Previously, the biosynthetic pathway of the immunosuppressive agent caerulomycin A (CRM A) from the marine actinomycete Actinoalloteichus cyanogriseus WH1-2216-6 has been identified, and the critical role of the (S)-selective ω-transaminase CrmG in the biosynthesis of CRM A has been reported. CrmG catalyzes amino acceptor caerulomycin M (CRM M) transformation to caerulomycin N (CRM N). Moreover, the activity of CrmG is insensitive to inhibition from ketone α-ketoglutarate or pyruvate.

The crystal structures of CrmG in complex with amino donor l-Gln, l-Glu, or l-Ala in P1 space group were determined to resolution 2.35, 2.25, and 2.20 Å, respectively. For these three crystal structures, each asymmetric unit contains two dimers. In the structures of CrmG with l-Glu or l-Ala, clear electron density was observed between the N atoms of those amino donors and the C4′ atom of PLP, indicating that we have captured the external aldimine for these amino acids. In the structure of CrmG with PLP-Glu, γ-carboxylate of the l-Glu portion not only forms a hydrogen bond with S372′ but also forms an additional salt bridge with K210. Based on these three crystal structures, amino donors l-Glu, l-Gln, and l-Ala exhibit strong, moderate, and weak binding to CrmG, respectively, due to side chain differences. These corroborate well with our kinetic data that, Km value for l-Glu, l-Gln, and l-Ala toward CrmG is 80.02, 182.70, and 405.10 μM, respectively. Moreover, in the case of l-Glu, which forms stronger interactions with the active site of CrmG than l-Ala, the corresponding by-product α-ketoglutarate also exhibits very weak inhibitory potential with a Ki value of 145.9 mM. The energy profile for CrmG catalyzing l-Glu deamination was calculated based on the crystal structures of PLP-bound CrmG and l-Glu-bound CrmG; the energy profile for CrmG catalyzing CRM M amination was calculated based on structures of PMP-bound CrmG and CRM M-bound CrmG. CrmG catalyzing l-Glu deamination is an exothermic reaction with calculated reaction enthalpy of −33.5 kcal/mol, and CRM M amination is endothermic with calculated reaction enthalpy of 11.5 kcal/mol.

>[4x]MTHPSGEPVYADAVLNGWLTSMGLGVEYVRAEGNTVYYLDDEGREVPVLDHACGFGSLIFGHNHPEIIAHAKAALDAGTVVHAQLSRQPRANQISRILNDIMRRETGRDDRYNAIFANSGAEANEICMKHAELERQERITALFAEIDAELDTAREALTTGTATLDTASLPLVGGGAGDVDGVIADIHRHNDERRAERPLFLTLDGSFHGKLVGSIQLTQNEPWRTPFTALSSPARFLPADEPELIGKIVEDERRSVLTLSLDKDTVRVVERDFPVVAAIFVEPVRGGSGMKTVTPELAEELHRLRDTLGCPLVVDEVQTGIGRTGAFFGSALLGIRGDYYTLAKAIGGGIVKNSVALIRQDRFLPAMEVIHSSTFAKDGLSASIALKVLEMVEADGGRVYQRVRERGQRLEAMLESVRADHSDVVSAVWGTGLMLALELRDQSNATSQAIREKAAHGFLGYVLAGFLLREHHIRVLPAGPRSGFLRFSPSLYITDEEIDRTETALRSLFTALRDQDGDRLVLS> MHHHHHHSSGRENLYFQGSVFGVPLTVNVQRTGQPLPQSIQQAMRYLRNHCLDQVGLFRKSGVKSRIQALRQMNEGAIDCVNYEGQSAYDVADM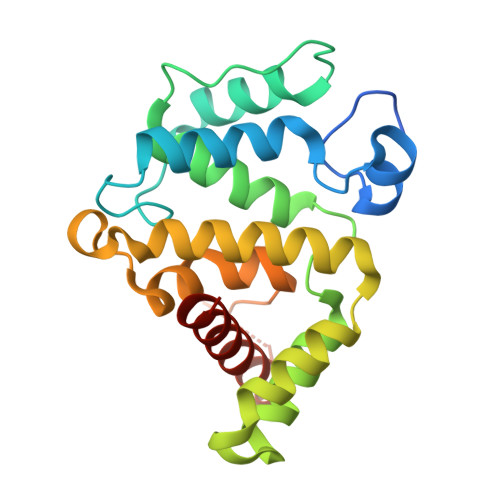LKQYFRDLPEPLMTNKLSETFLQIYQYVPKDQRLQAIKAAIMLLPDENREVLQTLLYFLSDVTAAVKENQMTPTNLAVCLAPSLFHLNTLKRENSSPRVMQRKQSLGKPDQKDLNENLAATQGLAHMIAECKKL> MNQEEAIFRSADMTYVQLYIPLEVIREVTFLLGKMSVFMVMDLNKDLTAFQRGYVNQLRRFDEVERMVGFLNEVVEKHAAETWKYILHIDDEGNDIAQPDMADLINTMEPLSLENVNDMVKEITDCESRARQLDESLDSLRSKLNDLLEQRQVIFECSKFIEVNPGIAGRATNPEIEQEERDVDEFRMTPDDISETLSDAFSFDDETPQDRGALGNDLTRNQSVEDLSFLEQGYQHRYMITGSIRRTKVDILNRILWRLLRGNLIFQNFPIEEPLLEGKEKVEKDCFIIFTHGETLLKKVKRVIDSLNGKIVSLNTRSSELVDTLNRQIDDLQRILDTTEQTLHTELLVIHDQLPVWSAMTKREKYVYTTLNKFQQESQGLIAEGWVPSTELIHLQDSLKDYIETLGSEYSTVFNVILTNKLPPTYHRTNKFTQAFQSIVDAYGIATYKEINAGLATVVTFPFMFAIMFGDMGHGFILFLMALFLVLNERKFGAMHRDEIFDMAFTGRYVLLLMGAFSVYTGLLYNDIFSKSMTIFKSGWQWPSTFRKGESIEAKKTGVYPFGLDFAWHGTDNGLLFSNSYKMKLSILMGYAHMTYSFMFSYINYRAKNSKVDIIGNFIPGLVFMQSIFGYLSWAIVYKWSKDWIKDDKPAPGLLNMLINMFLAPGTIDDQLYSGQAKLQVVLLLAALVCVPWLLLYKPLTLRRLNKNGGGGRPHGYQSVGNIEHEEQIAQQRHSAEGFQGMIISDVASVADSINESVGGGEQGPFNFGDVMIHQVIHTIEFCLNCISHTASYLRLWALSLAHAQLSSVLWDMTISNAFSSKNSGSPLAVMKVVFLFAMWFVLTVCILVFMEGTSAMLHALRLHWVEAMSKFFEGEGYAYEPFSFRAIIEDYKDHDGDYKDHDIDYKDDDDK;> MVFGQLYALFIFTLSCCISKTVQADSSKESSSFISFDKESNWDTISTISSTADVISSVDSAIAVFEFDNFSLLDNLMIDEEYPFFNRFFANDVSLTVHDDSPLNISQSLSPIMEQFTVDELPESASDLLYEYSLDDKSIVLFKFTSDAYDLKKLDEFIDSCLSFLEDKSGDNLTVVINSLGWAFEDEDGDDEYATEETLSHHDNNKGKEGDDDILSSIWTEGLLMCLIVSALLLFILIVALSWISNLDITYGALEKSTNPIKKNN;> MNKESKDDDMSLGKFSFSHFLYYLVLIVVIVYGLYKLFTGHGSDINFGKFLLRTSPYMWANLGIALCVGLSVVGAAWGIFITGSSMIGAGVRAPRITTKNLISIIFCEVVAIYGLIIAIVFSSKLTVATAENMYSKSNLYTGYSLFWAGITVGASNLICGIAVGITGATAAISDAADSALFVKILVIEIFGSILGLLGLIVGLLMAGKASEFQ;> MEGVYFNIDNGFIEGVVRGYRNGLLSNNQYINLTQCDTLEDLKLQLSSTDYGNFLSSVSSESLTTSLIQEYASSKLYHEFNYIRDQSSGSTRKFMDYITYGYMIDNVALMITGTIHDRDKGEILQRCHPLGWFDTLPTLSVATDLESLYETVLVDTPLAPYFKNCFDTAEELDDMNIEIIRNKLYKAYLEDFYNFVTEEIPEPAKECMQTLLGFEADRRSINIALNSLQSSDIDPDLKSDLLPNIGKLYP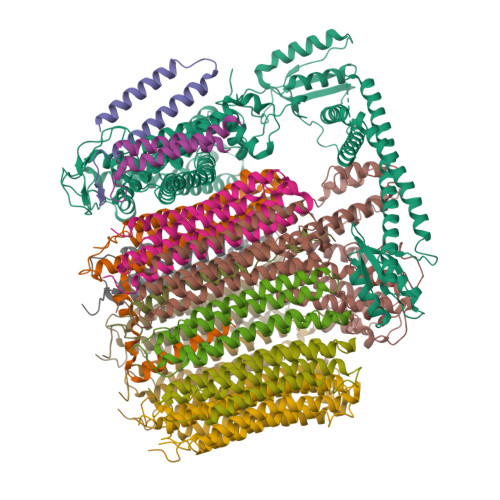LATFHLAQAQDFEGVRAALANVYEYRGFLETGNLEDHFYQLEMELCRDAFTQQFAISTVWAWMKSKEQEVRNITWIAECIAQNQRERINNYISVY;> MSSFYTVVGVFIVVSAMSVLFWIMAPKNNQAVWRSTVILTLAMMFLMWAITFLCQLHPLVAPRRSDLRPEFAE;> MRPVVSTGKAWCCTVLSAFGVVILSVIAHLFNTNHESFVGSINDPEDGPAVAHTVYLAALVYLVFFVFCGFQVYLARRKPSIELR;>[8x]MTELCPVYAPFFGAIGCASAIIFTSLGAAYGTAKSGVGICATCVLRPDLLFKNIVPVIMAGIIAIYGLVVSVLVCYSLGQKQALYTGFIQLGAGLSVGLSGLAAGFAIGIVGDAGVRGSSQQPRLFVGMILILIFAEVLGLYGLIVALLLNSRATQDVVC;> MSTQLASNIYAPLYAPFFGFAGCAAAMVLSCLGAAIGTAKSGIGIAGIGTFKPELIMKSLIPVVMSGILAIYGLVVAVLIAGNLSPTEDYTLFNGFMHLSCGLCVGFACLSSGYAIGMVGDVGVRKYMHQPRLFVGIVLILIFSEVLGLYGMIVALILNTRGSE> GGHHHHHHGSENLYFQGACPSQCSCSGTTVDCSGKSLASVPTGIPTTTQVLGLSSNQITKLEPGVFDSLVNLQILVLYQNQLTTLPAGVFDRLINLKELYFSNNQLTSLPAGVFDK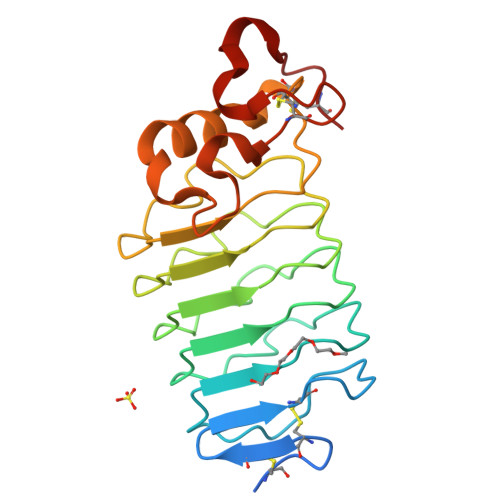LTQLTRLELQTNQLKSIPRGAFDNLKSLTNIYLFNNPWDCECSDILYLKNWIVQHASIVNPDGHGGVDNVKCSGTNTPVRAVTEASTSPSKCP> MAEAGLRGWLLWALLLRLAQSEPYTTIHQPGYCAFYDECGKNPELSGSLMTLSNVSCLSNTPARKITGDHLILLQKICPRLYTGPNTQACCSAKQLVSLEASLSITKALLTRCPACSDNFVNLHCHNTCSPNQSLFINVTRVAQLGAGQLPAVVAYEAFYQHSFAEQSYDSCSRVRVPAAATLAVGTMCGVYGSALCNAQRWLNFQGDTGNGLAPLDITFHLLEPGQAVGSGIQPLNEGVARCNESQGDDVATCSCQDCAASCPAIARPQALDSTFYLGQMPGSLVLIIILCSVFAVVTILLVGFRVAPARDKSKMVDPKKGTSLSDKLSFSTHTLLGQFFQGWGTWVASWPLTILVLSVIPVVALAAGLVFTELTTDPVELWSAPNSQARSEKAFHDQHFGPFFRTNQVILTAPNRSSYRYDSLLLGPKNFSGILDLDLLLELLELQERLRHLQVWSPEAQRNISLQDICYAPLNPDNTSLYDCCINSLLQYFQNNRTLLLLTANQTLMGQTSQVDWKDHFLYCANAPLTFKDGTALALSCMADYGAPVFPFLAIGGYKGKDYSEAEALIMTFSLNNYPAGDPRLAQAKLWEEAFLEEMRAFQRRMAGMFQVTFMAERSLEDEINRTTAEDLPIFATSYIVIFLYISLALGSYSSWSRVMVDSKATLGLGGVAVVLGAVMAAMGFFSYLGIRSSLVILQVVPFLVLSVGADNIFIFVLEYQRLPRRPGEPREVHIGRALGRVAPSMLLCSLSEAICFFLGALTPMPAVRTFALTSGLAVILDFLLQMSAF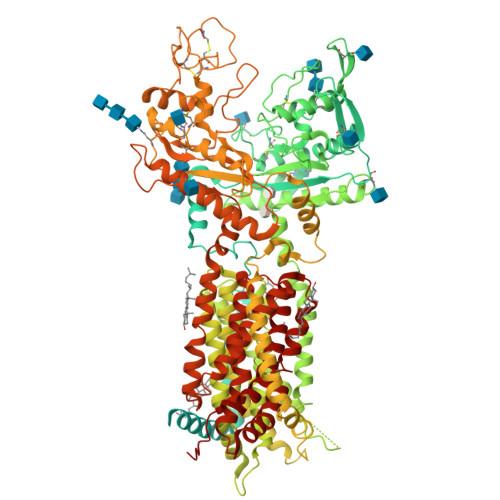VALLSLDSKRQEASRLDVCCCVKPQELPPPGQGEGLLLGFFQKAYAPFLLHWITRGVVLLLFLALFGVSLYSMCHISVGLDQELALPKDSYLLDYFLFLNRYFEVGAPVYFVTTLGYNFSSEAGMNAICSSAGCNNFSFTQKIQYATEFPEQSYLAIPASSWVDDFIDWLTPSSCCRLYISGPNKDKFCPSTVNSLNCLKNCMSITMGSVRPSVEQFHKYLPWFLNDRPNIKCPKGGLAAYSTSVNLTSDGQVLASRFMAYHKPLKNSQDYTEALRAARELAANITADLRKVPGTDPAFEVFPYTITNVFYEQYLTILPEGLFMLSLCLVPTFAVSCLLLGLDLRSGLLNLLSIVMILVDTVGFMALWGISYNAVSLINLVSAVGMSVEFVSHITRSFAISTKPTWLERAKEATISMGSAVFAGVAMTNLPGILVLGLAKAQLIQIFFFRLNLLITLLGLLHGLVFLPVILSYVGPDVNPALA>MFSGIKGPNPSDLKGPELRILIVHARWNLQAIEPLVKGAVETMIEKHDVKLENIDIESVPGSWELPQGIRASIARNTYDAVIGIGVLIKGSTMHFEYISEAVVHGLMR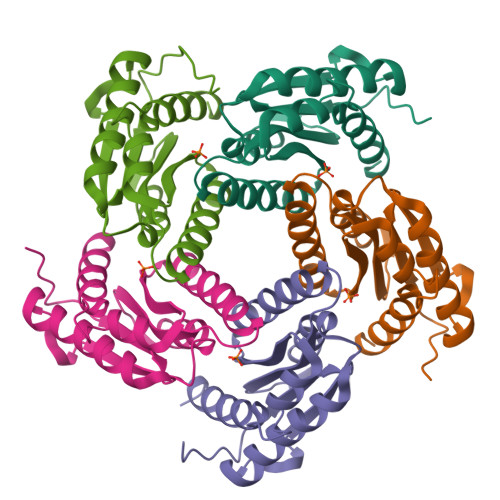VGLDSGVPVIFGLLTVLNEEQALYRAGLNGGHNHGNDWGSAAVEMGLKALY[5x]>[2x]GDKCKKTTTCEPLKYNICLGSVLPYA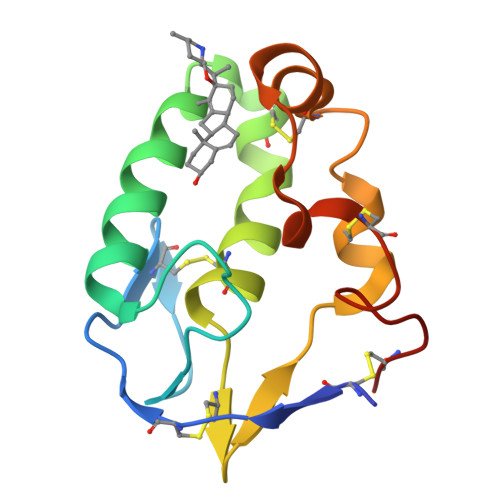LTSTVLAEDSSSQDEVHDKLSLWSGLRNAPRCWDAIRPLLCAVYMPKCEGGKVELPSQGLCQTTRVPCAIVARERGWPDFLKCTTDYFPEGCPNE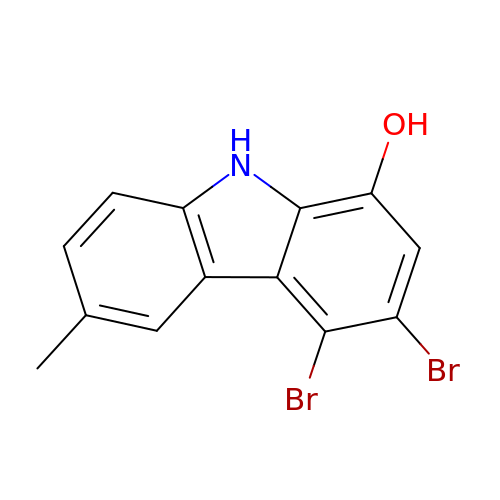3,6-dibromo-1-(hydroxymethyl)carbazole | C13 H9 Br2 N O | LFOHIKGNXVHWSB-UHFFFAOYSA-N NoVs recognize specific glycan ligands as host attachment factors or receptors for infection. NoVs interact with HBGAs or other glycans through their capsid protrusions that are built by the dimeric protruding (P) domain of NoV capsid protein (VP1). Genogroup II (GII) noroviruses consist of human noroviruses (huNoVs) that generally bind histo-blood group antigens (HBGAs) as host factors and three porcine norovirus (porNoV) genotypes (GII.11/18/19) that form a genetic lineage lacking HBGA-binding ability. In this study, we solved the P protein crystal structures of a GII.11 porNoV (VA34) that was isolated from pig caecum contents in 1997 in Japan and a close-related GII.3 huNoV (TV24) that was isolated in 1977 in the USA, representing one of the earliest huNoV isolates, focusing on their HBSs compared with the previously known ones.

The crystal structure of the native GII.3 huNoV TV24 P protein was solved to 2.6 Å resolution, revealing P protein homodimers in the crystallographic asymmetric unit. All P protein residues were modelled in the electron density map, except for 13 amino acids from 295 to 307 in the B-loop (see below), due to the disorder of this highly flexible long loop. The TV24 P dimer exhibits a typical NoV P dimer global structure. Interestingly, VA34 and TV24 P proteins share the longest B-loop compared with other GII NoVs, leading to the observed disorders in the crystallography and thus the unknown conformation of 13 and 12 residues of this loop. The two P proteins also share the small T-loop with an α-helix extruding out of the flat surface (Figure 6(C–F), Figure S3). The TV24 P protein bound secretor positive types O, A, and B human saliva samples weakly with optical density (OD) readings up to ∼0.4. All three P protein mutants with a single-residue mutation at the HBS wiped out the HBGA binding capability to all type O, A, B, and non-secretor saliva samples completely or nearly completely, indicating the requirements of the three amino acids individually for the structural and functional integrity of the TV24 HBS.

>GPLGSSKTKPFTLPILTISEMSNSRFPVPIDSLHTSPTENIVVQCQNGRVTLDGELMGTTQLLPSQICAFRGTLTRSTSRASDQADTPTPRLFNYYWHIQLDNLNGTPYDPAEDIPAPLGTPDFRGKVFGVASQRNPDSTTRAHEAKVDTTSGRFTPKLGSLEITTESDDFDPNQPTKFTPVGVGVDNEAEFQQWSLPNYSGQFTHNMNLAPAVAPNFPGEQLLFFRSQLPSSGGRSNGVLDCLVPQEWVQHFYQESAPAQTQVALVRYVNPDTGRVLFEAKLHKLGFMTIAKNGDSPITVPPNGYFRFESWVNPFYTLAPMGTGNG[4x]>MDRLKALVDAAVQPVMKANDIPGLAVAISLKGEPHYFSYGLASKEDGRRVTPETLFEIGSVSKTFTATLAGYALTQDKMRLDDRASQHWPALQGSRFDGISLLDLATYTAGGLPLQFPDSVQKDQAQIRDYYRQWQPTYAPGSQRLYSNPSIGLFGYLAARSLGQPFERLMEQQVFPALGLEQTHLDVPEAALAQYAQGYGKDDRPLRVGPGPLDAEGYGVKTSAADLLRFVDANLHPERLDRPWAQALDATHRGYYKVGDMTQGLGWEAYDWPISLKRLQAGNSTPMALQPHRIARLPAPQALEGQRLLNKTGSTNGFGAYVAFVPGRDLGLVILANRNYPNAERVKIAYA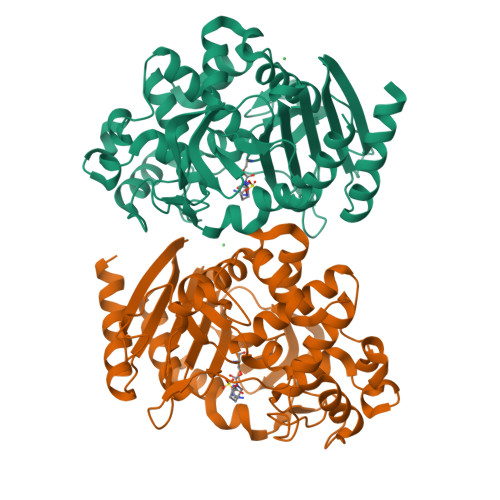ILSGL[2x]>[4x]MGGSSGGGVSYRSGGESDVELEDYEVDDFRDGIVESRGNRFNPLTNFLGLDFAGGSGGKFTVINGIRDISRGSIVHPDNRWYKAWTMFILIWALYSSFFTPLEFGFFRGLPENLFILDIAGQIAFLVDIVLTFFVAYRDSRTYRMIYKRSSIALRYLKSTFIIDLLACMPWDIIYKAAGEKEEVRYLLLIRLYRVHRVILFFHKMEKDIRINYLFTRIVKLIFVELYCTHTAACIFYYLATTLPASQEGYTWIGSLKLGDYSYSKFREIDLWTRYTTSMYFAVVTMATVGYGDIHAVNMREMIFAMVYISFDMILGAYLIGNMTALIVKGSKTERFRDKMADIMRYMNRNKLGRNIRGQITGHLRLQYESSYTEAAVLQDIPVSIRAKIAQTLYLPYIEKVPLFRGCSSEFINQIVIRLHEEFFLPGEVIMEQGSVVDQLYFVCHGVLEEIGITKDGSEEIVAVLQPDHSFGEISILCNIPQPYTVRVAELCRILRLDKQSFMNILEIFFHDGRRILNNLLEGKESNVRIKQLESDITFHISKQEAELALKLNSAAFYGDLYQLKSLIRAGGDPNKTDYDGRSPLHLAASRGYEDITLYLIQESVDVNIKDKLGSTPLLEAIKNGNDRVAALLVKEGATLNIENAGTFLCTVVAKGDSDFLKRLLSNGIDPNSKDYDHRTPLHVAASEGFYVLAIQLVEASANVLAKDRWGNTPLDEALGCGNKMLIKLLEDAKNSQISSFPSGSKEPKDKVYKKKCTVYFSHPGDSKEKRRRGIVLWVPRSIEELIRTAKEQLNVPEASCVLSEDEAKIIDVDLISDGQKLYLAVET

Among these channels, the Stelar K+ outward rectifier channel (SKOR) functions as a K+ efflux channel for long-distance distribution of K+ from roots to the upper parts of the plant. Interestingly, SKOR contains an intracellular ankyrin repeat (ANK) domain, which is absent in all the depolarization-activated K+ channels with known structure. Each protomer can be arbitrarily divided into four layers along the central axis: a transmembrane domain (TMD) comprising six transmembrane α-helices designated as S1–S6, a gating ring formed by the C-linker, a cytoplasmic domain homologous with the cyclic nucleotide-binding domain (CNBD), and an ANK domain. Unlike the canonical potassium channel, SKOR does not adopt a C4 but a C2 symmetry, which occurs in the C-linker, CNBD and ANK domain.

After extensive 3D classification and refinement, two final maps of SKOR (named SKORwt1 and SKORwt2) with global resolutions of 3.1 Å and 3.5 Å were obtained. Interestingly, the overall architectures of both SKORwt1 and SKORwt2 do not adopt canonical C4 symmetry but exhibit a dramatic reduction of symmetry from C4 to C2. In the structure of SKORwt1, four ANK domains are divided into two pairs; the two ANK domains in each pair form close contacts with each other, and a gap is present between the two pairs, resulting in a C2 symmetry. As a result of this asymmetry, the inter-CNBD interactions around the channel ring differ considerably. Compared to KAT1, SKORwt1 exhibits a significant rotation in the C-linker and CNBD. Moreover, the distinct extent of rotation in the adjacent subunits leads to breaking of C4 symmetry in SKOR. Superposition of the structures of the ANKs from SKORwt1 and TRPA1 reveals that repeats 1 and 2 in SKOR are assembled similarly to those in TRPA1, whereas repeats 4, 5 and 6 display a clockwise rotation relative to TRPA1 due to the lack of β-hairpin in repeat 3. The packing of ANKs in SKORwt2 is different from that in SKORwt1. Notably, as a depolarization-activated channel, SKOR was expected to adopt an open conformation in vitro (0 mV) like Kv1.311 and hERG channels, but both SKORwt1 and SKORwt2 were found to be in a closed state. The ANK-induced symmetry reduction may be responsible for this closed state.2-deoxy-2-(ethanethioylamino)-beta-D-glucopyranose | C8 H15 N O5 S | 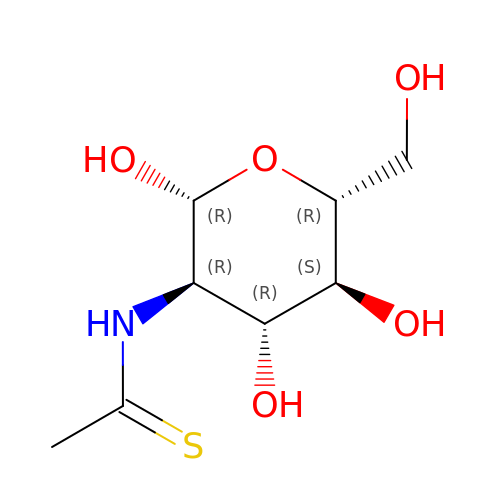BIHKKHHUWVSGSD-FMDGEEDCSA-N> SRVKSLKKSLRQSFRR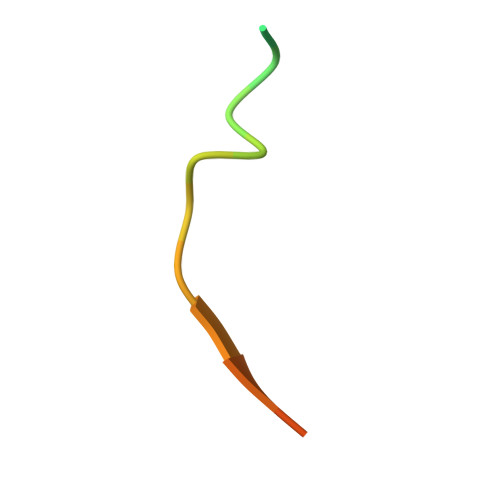MRKS>MPMVLLECDKDIPERQKHIYLKAPNEDTREFLPIANAATIPGTLSERGCAFCGAKLVIGGVLKDTIQMIHGPLGCAYDTWHTKRYPTDNGHFNMKYVWSTDMKESHVVFGGEKRLEKSMHEAFDEMPDIKRMIVYTTCPTALIGDDIKAVAKKVMKDRPDVDVFTVECPGFSGVSQSKGHHVLNIGWINEKVETMEKEITSEYTMNFIGDFNIQGDTQLLQTYWDRLGIQVVAHFTGNGTYDDLRCMHQAQLNVVNCARSSGYIANELKKRYGIPRLDIDSWGFNYMAEGIRKICAFFGIEEKGEELIAEEYAKWKPKLDWYKERLQGKKMAIWTGGPRLWHWTKSVEDDLGVQVVAMSSKFGHEEDFEKVIARGKEGTYYIDDGNELEFFEIIDLVKPDVIFTGPRVGELVKKLHIPYVN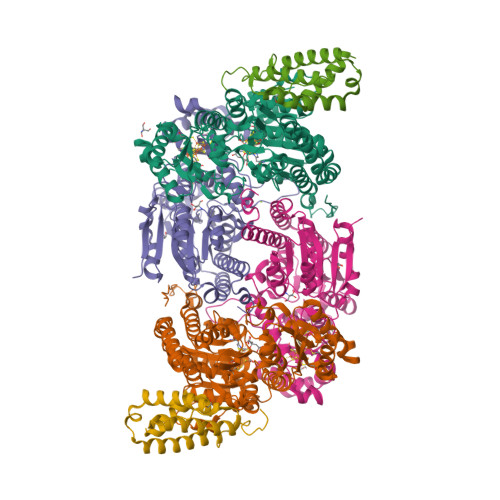GHGYHNGPYMGFEGFVNLARDMYNAVHNPLRHLAAVDIRDKSQTTPVIVRGAA[2x];>[2x]MSNCELTVLKPAEVKLSPRDREGIINPMYDCQPAGAQYAGIGIKDCIPLVHGGQGCTMFVRLLFAQHFKENFDVASTSLHEESAVFGGAKRVEEGVLVLARRYPNLRVIPIITTCSTEVIGDDIEGSIRVCNRALEAEFPDRKIYLAPVHTPSFKGSHVTGYAECVKSVFKTITDAHGKGQPSGKLNVFPGWVNPGDVVLLKRYFKEMDVEANIYMDTEDFDSPMLPNKSIETHGRTTVEDIADSANALATLSLARYEGNTTGELLQKTFAVPNALVNTPYGIKNTDDMLRKIAEVTGKEIPESLVRERGIALDALADLAHMFFANKKVAIFGHPDLVLGLAQFCMEVELEPVLLLIGDDQGNKYKKDPRIEELKNTAHFDIEIVHNADLWELEKRINAGLQLDLIMGHSKGRYVAIEANIPMVRVGFPTFDRAGLYRKPSIGYQGAMELGEMIANAMFAHMEYTRNKEWILNTW;>[2x]MSQSHLDDLFAYVEERCLWQFFSRTWDREENIEGVLNQVGRLLTGQEPLRGTPQERLFYADALAMANDVRERFPWASQVNKEEIEFLLDGLKSRLVDVTITRSTNRELNHHLY> MTQVLVRNGIQAVGDGLTSLIIVGKKSVLKNVTFEGKFKEVAQKFVTDGDSWNSMISRIPASGRHPLHYELAHLITVPDASSRGNTPTNAHSIYKELKPINYPEDTKNVHFVLFAEYPDVLSHVAAIARTFCKFSMKTSGIRELNVNIDVVCDKLTNEDAVFLTDLSESVRETARLIDTPANILTTDALVDEAVKVGNATGSKITVIRGEELLKAGFGGIYHVGKAGPTPPAFVVLSHEVPGSTEHIALVGKGVVYDTGGLQIKTKTGMPNMKRDMGGAAGMLEAYSALVKHGFSQTLHACLCIVENNVSPIANKPDDIIKMLSGKTVEINNTDAEGRLILADGVFYAKETLKATTIFDMATLTGAQAWLSGRLHGAAMTNDEQLENEIIKAGKASGDLVAPMLF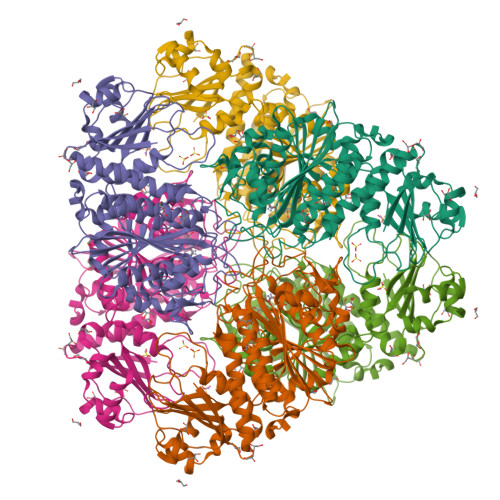APDLFFGDLKSSIADMKNSNLGKMDGPPSAVAGLLIGAHIGFGEGLRWLHLDIAAPAEVGDRGTGYGPALFSTLLGKYTSVPMLKQ>GNLPPEKKWLGTPIEEMRKMPRCGIHLPSLRPSASHTVTVRVDLLRAGEVPKPFPTHYKDLWDNKHVKMPCSEQNLYPVEDENGERTAGSRWELIQTALLNKFTRPQNLKDAILKYNVAYSKKWDFTALVDFWDKVLEEAEAQHLYQSILPDMVKIALCLPNICTQPIPLLKQKMNHSVTMSQEQIASLLANAFFCTFPRRNAKMKSEYSSYPDINFNRLFEGRSSRKPEKLKTLFCYFRRVTEKKPTGLVTFTRQSLEDFPEWERCEKPLTRLHVTYEGTIEGNGRGMLQVDFANRFVGGGVTGAGLVQENIRFLINPELIVSRLFTEVLDHNECLIITGTEQYSEYTGYAETYRWARSHEDGSEKDDWQRRCTEIVAIDALHFRRYLDQFVPEKVRRELNKAYCGFLRPGVPSENLSAVATGNWGCGAFGGDARLKALIQILAAAAAERDVVYFTFGDSELMRDIYSMHTFLTERKLDVGKVYKLLLRYYNEECRNCSTPGPDIKLYPFIYHAVESSAET[2x]

Reversal of PARylation is predominantly carried out by poly(ADP-ribose) glycohydrolase (PARG) in nucleus and cytosol, whereas ADP-ribosylhydrolase 3 (ARH3) may play a role in mitochondrial PAR degradation. PARG comprises an N-terminal regulatory/targeting domain and a C-terminal catalytic domain. The mouse PARG catalytic domain has a bean-shaped structure, with the active site in a deep cleft in the middle on the abdominal side.

To understand what caused the activity difference between the mPARG E748N/Q and E749N/Q mutants, we solved the crystal structures of these mPARG mutants. Interestingly, while E748N and E749N mutants were completely dead, both E748Q and E749Q mutants still retained residual PARG activities. In contrast, the signature loops in E748N and E749N mutants have significantly different conformation from the wild type PARG. In wild-type PARG structure, Cβ and Cγ of both E748 and E749 residues are semi-buried. Mutation to Asn, which has both Cγ and Nγ linked to Cβ causes a spatial collision. Therefore, the conformation changes in this catalytic loop completely abolish activity of mPARG E748N and E749N mutants. To study the enzymatic mechanism of mPARG, we tried to soak the catalytic residue Glu748, Glu749 mutants E748N, E748Q, E749N and E749Q with the iso-ADPr, which may be the smallest PARG substrate containing the α(1→2) ribose-ribose glycosidic bond to be cleaved by PARG. In all above four PARG mutant crystal structures, we were not able to observe the electron density for iso-ADPr at the “active” site of mPARG. For E748N and E749N mutants, this may result from the conformational change in the active site associated with the mutation. Our work revealed precisely how some of the PARG mutations (e.g. E748N, E749N) disrupt the PARG activity through significant conformational changes in the PARG active site.>[4x]GPGSN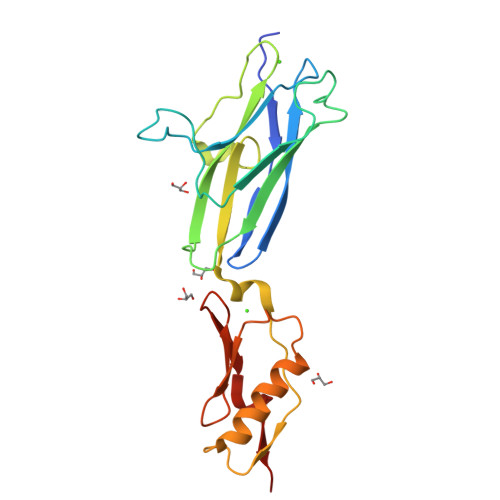DTEAPQVKSGDYVVYRGESFEYYAEITDNSGQVNNVVVRNVELDKKTNMPYLTPDWLKYSTDNLGQPGNATVENPLRTKLYGNVPLDTVVGIYTRYIVATDPANNTTRMIQNPNRDGLERFVLTVKSQNEKYDPADPSVTYVNNLSNLSTSERDAVAAAVRAANPSLPSAAKITVSQNGTVTITYPDRSTDTIPANRVVKDLQIS>SDELSFTINNFVPNEADLLFQGEASVSSTGVLQLTKVENGQPQKYSVGRALYAAPVRIWGNTTGSVASFSTSFTFVVKAPNPDITSDGLAFYLAPPDSQIPSGSVSKYLGLFNNSNSDSSNQIVAVEFDTYFAHSYDPWDPNYRHIGIDVNGIESIKTVQWDWINGGVAFATITYLAPNKTLIASLVYPSNQTTFSVAASVDL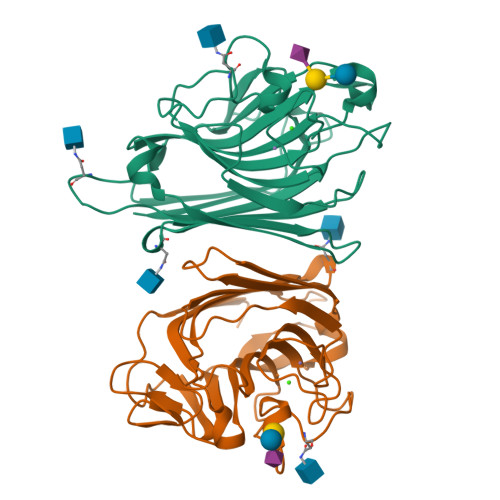KEILPEWVRVGFSAATGYPTEVETHDVLSWSFTSTL[2x]>MALCEAEEAPPASSTPHVVGSRFNWKLFWQFLHPHLLVLGVAVVLALGAALVNVQIPLLLGQLVEVVAKYTRDHVGSFMTESQNLSTHLLILYGVQGLLTFGYLVLLSHVGERMAVDMRRALFSSLLRQDITFFDANKTGQLVSRLTTDVQEFKSSFKLVISQGLRSCTQVAGCLVSLSMLSTRLTLLLMVATPALMGVGTLMGSGLRKLSRQCQEQIARAMGVADEALGNVRTVRAFAMEQREEERYGAELEACRCRAEELGRGIALFQGLSNIAFNCMVLGTLFIGGSLVAGQQLTGGDLMSFLVASQTVQRSMANLSVLFGQVVRGLSAGARVFEYMALNPCIPLSGGCCVPKEQLRGSVTFQNVCFSYPCRPGFEVLKDFTLTLPPGKIVALVGQSGGGKTTVASLLERFYDPTAGVVMLDGRDLRTLDPSWLRGQVVGFISQEPVLFGTTIMENIRFGKLEASDEEVYTAAREANAHEFITSFPEGYNTVVGERGTTLSGGQKQRLAIARALIKQPTVLILDEATSALDAESERVVQEALDRASAGR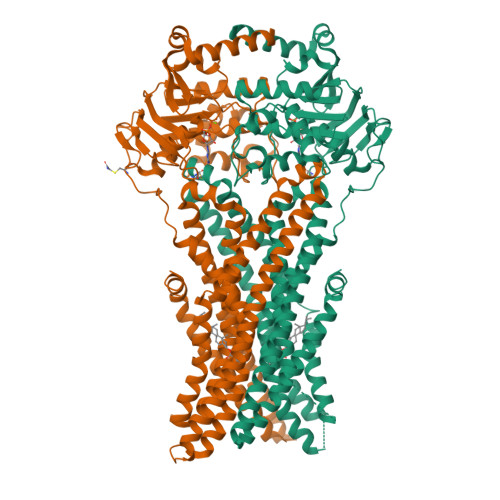TVLVIAHRLSTVRGAHCIVVMADGRVWEAGTHEELLKKGGLYAELIRRQALDAAENLYFQ[8x]N-(5-benzyl-1,3-thiazol-2-yl)-2-[(4,6-dimethylpyrimidin-2-yl)sulfanyl]acetamide | C18 H18 N4 O S2 | 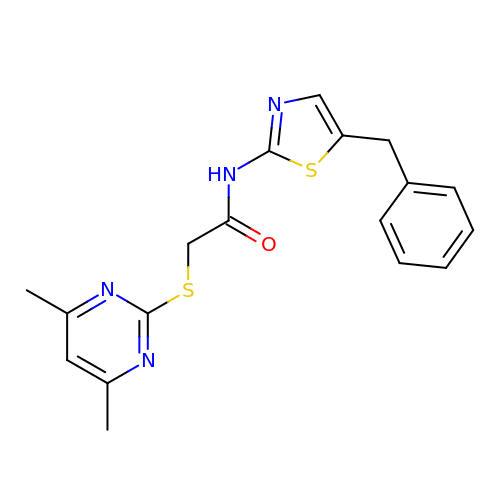LHMBJRUBDQYYSV-UHFFFAOYSA-N>[2x]MATLTAKNLAKAYKGRRVVEDVSLTVNSGEIVGLLGPNGAGKTTTFYMVVGIVPRDAGNIIIDDDDISLLPLHARARRGIGYLPQEASIFRRLSVYDNLMAVLQIRDDLSAEQREDRANELMEEFHIEHLRDSMGQSLSGGERRRVEIARALAANPKFILLDEPFAGVDPISVIDIKRIIEHLRDSGLGVLITDHNVRETLAVCERAYIVSQGHLIAHGTPTEILQDEHVKRVYLGEDFRL;> MIIIRYLVRETLKSQLAILFILLLIFFCQKLVRILGAAVDGDIPANLVLSLLGLGVPEMAQLILPLSL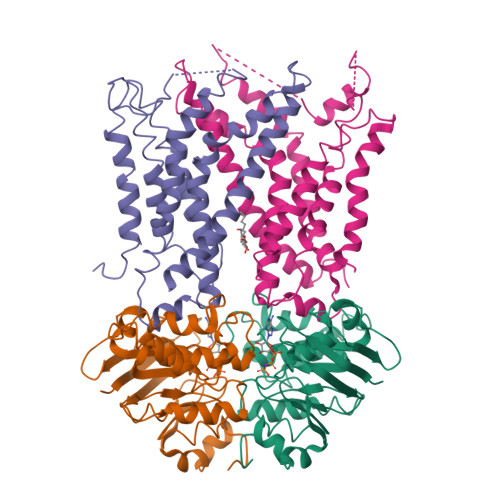FLGLLMTLGKLYTESEITVMHACGLSKAVLVKAAMILAVFTAIVAAVNVMWAGPWSSRHQDEVLEEAKANPGMAALAQGQFQQATNGSSVLFIESVDGSDFKDVFLAQIRPKGNARPSVVVADSGHLTQLRDGSQVVTLNQGTRFEGTALLRDFRITDFQDYQAIIGHQAVALDPNDTDQMDMRTLWNTDTDRARAELNWRITLVVTVFMMALMVVPLSVVNPRQGRVLSMLPAMLLYLLFFLIQTSLKSNGGKGKLDPTLWMWTVNLIYLALAIVLNLWDTVFVRRLRASFSRKGAV;> MQPFGVLDRYIGKTIFTTIMMTLFMLVSLSGIIKFVDQLKKAGQGSYDALGAGMYTLLSVPKDVQIFFPMAALLGALLGLGMLAQRSELVVMQASGFTRMQVALSVMKTAIPLVLLTMAIGEWVAPQGEQMARNYRAQAMYGGSLLSTQQGLWAKDGNNFVYIERVKGDEVLGGISIYAFNENRRLQSVRYAATAKFDPEHKVWRLSQVDESDLTNPKQITGSQTVSGTWKTDLTPDKLGVVALDPDALSISGLHNYVKYLKSSGQDAGRYQLNMWSKIFQPLSVAVMMLMALSFIFGPLRSVPMGVRVVTGISFGFVFYVLDQIFGPLTLVYGIPPIIGALLPSASFFLISLWLLMRKS>[2x]MFVTMNRIPVRPEYAEQFEEAFRQRARLVDRMPGFIRNLVLRPKNPGDPYVVMTL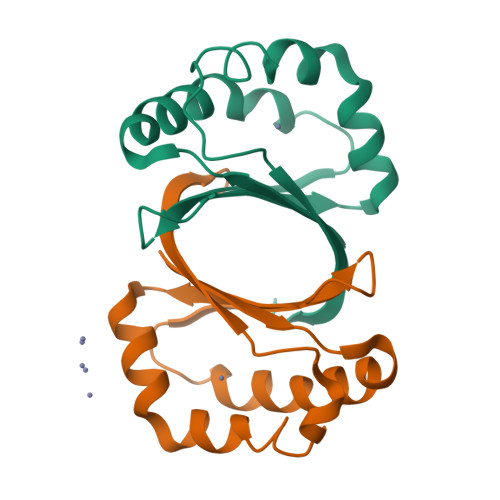WESEEAFRAWTESPAFKEGHARSGTLPKEAFLGPNRLEAFEVVLDSEGRDG3-[[6-(cyclohexylmethoxy)-9~{H}-purin-2-yl]amino]benzamide | C19 H22 N6 O2 | 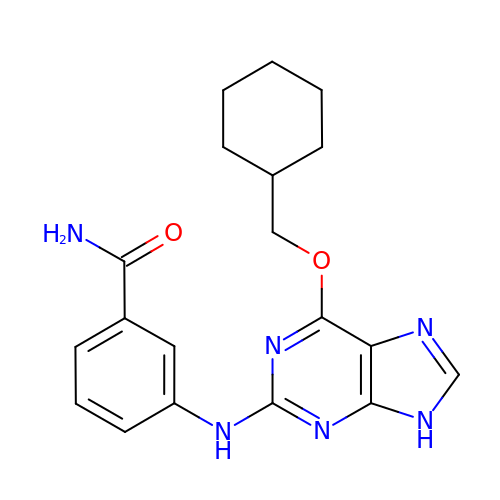XAOVCENYRWWHPR-UHFFFAOYSA-N Here we report a structural and functional analysis for an epimerase, KasQ, that primes KSM biosynthesis rather than the previously proposed KasF/H, which instead acts as an acetyltransferase, inactivating KSM. Our biochemical and biophysical analysis determined that KasQ converts UDP-GlcNAc to UDP-ManNAc as the initial step in the biosynthetic pathway. To better understand the catalytic mechanism of KasQ, we solved crystal structures of KasQ for the wild type (WT) and its complexes with UDP or UDP-Glc in resolutions of 2.44 Å, 2.58 Å, and 2.09 Å, respectively. In brief, each monomer consists of two domains (N-terminal and C-terminal domains), in which each subdomain is made of a typical sandwich (αβα) architecture of a Rossmann fold.

As revealed above, UDP or UDP-Glc is bound to its binding site at the interface of the two domains. The superimposition of KasQ–UDP and KasQ–UDP-Glc with an RMSD of 0.29 Å for 332 Cα atoms suggested no apparent conformational differences as a result of binding from different ligands. The electron density of UDP or UDP-Glc is well defined and consistent in the substrate binding site. The UDP binding site is highly conserved among all non-hydrolyzing UDP-GlcNAc 2-epimerases: the guanidino side chain of Arg12 and the backbone of Leu267 are in close contact with the uracil O2 atom, likely due to hydrogen bonding (3.1 Å and 3.4 Å, respectively). The backbone of Leu267 is also in a hydrogen-bonding distance to the O4 atom (3.1 Å) and the N3 atom (2.7 Å) of the uracil base. The two hydroxyl groups of the ribose moiety are associated with Glu292 (2.8 Å and 2.6 Å) by hydrogen bonds. His209 may play a role in stabilizing UDP by interacting with its α-phosphate (3.1 Å) and β-phosphate (2.6 Å). Ser286, Gly287, and Gly289 are three highly conserved residues for molecular recognition, in which Ser286 interacts with α/β phosphate (2.7 Å/3.2 Å, respectively), Gly287 is in contact with the O1/O2 atom of β-phosphate (3.3 Å/3.1 Å, respectively), and Gly289 is associated with the O1 atom of β-phosphate (2.9 Å). In the KasQ–UDP complex, the carboxyl group of Glu32 makes an additional interaction with the Na+ ion. Of these, the binding affinity of UDP versus KasQ was shown to be 2–5-fold higher than that of the others, suggesting that UDP-sugar is most likely the physiological substrate for KasQ.

>HMALRVGIVYGTRPEAIKLAPLVLALDADPGFEPVIITTGQHRDMLDEINELFGLRPRHNLDIMRPGQRLSAMASRIVGELGDPLLDELVDVAVVQGDTSTAFAAAYAAACERIPVAHLEAGLRTGDRFEPFPEEINRRLITQLADLHFAPTADAAGNLLAEGVRSDDVYVTGNTVIDAMHLVLDRPGDSANRELDAFTEGRQTVLLTMHRRESWGIPMGRVAAAVAELCRSRPTLRFVIPLHPNPEVRRVFRSHLSSLTQVLLCEPLRYSEFIRLMHRAVLVLTDSGGVQEEAPTLGKPVLVLRDRTERPEGIAAGCARLVGTDPALIVKEVGRLLDDPEAYEAMRRPGIVCYGEGDAAARCLEALRERWLSSP[8x]> MGSSHHHHHHSSGLVPRGSSFPWFGMDIGGTLVKLSYFEPIDITAEEEQEEVESLKSIRKYLTSNVAYGSTGIRDVHLELKDLTLFGRRGNLHFIRFPTQDLPTFIQMGRDKNFSTLQTVLCATGGGAYKFEKDFRTIGNLHLHKLDELDCLVKGLLYIDSVSFNGQAECYYFANASEPERCQKMPFNLDDPYPLLVVNIGSGVSILAVHSKDNYKRVTGTSLGGGTFLGLCSLLTGCESFEEALEMASKGDSTQADKLVRDIYGGDYERFGLPGWAVASSFGNMIYK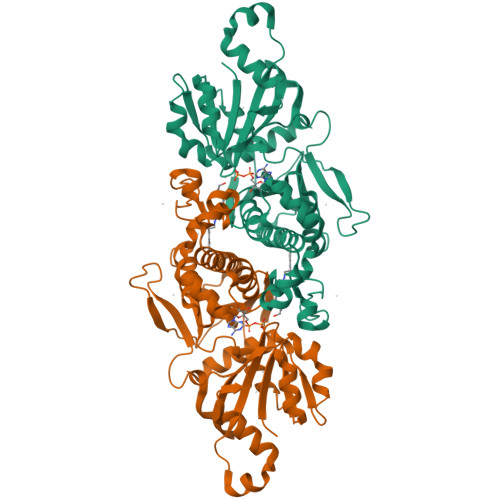EKRESVSKEDLARATLVTITNNIGSVARMCAVNEKINRVVFVGNFLRVNTLSMKLLAYALDYWSKGQLKALFLEHEGYFGAVGALLGLPNFSDD> EHLTIGFKVENAHDRILKTIKTHKLKNYIKESVNFLNSGLTKTNYLGSSNDNIELVDFQNIMFYGDAEVGDNQQPFTFILDTGSANLWVPSVKCTTAGCLTKHLYDSSKSRTYEKDGTKVEMNYVSGTVSGFFSKDLVTVGNLSLPYKFIEVIDTNGFEPTYTASTFDGILGLGWKDLSIGSVDPIVVELKNQNKIENALFTFYLPVHDKHTGFLTIGGIEERFYEGPLTYEKLNHDLYWQITLDAHVGNIMLEKANCIVDSGTSAITVPTD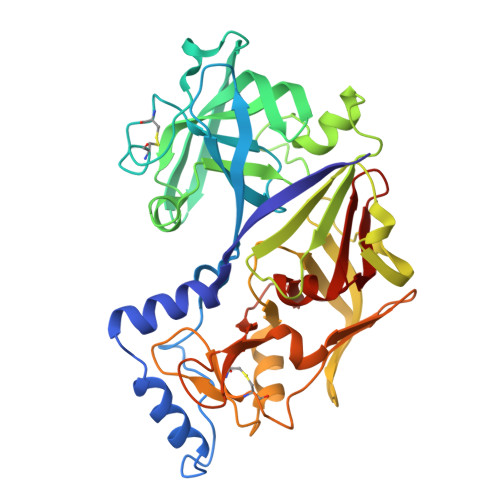FLNKMLQNLDVIKVPFLPFYVTLCNNSKLPTFEFTSENGKYTLEPEYYLQHIEDVGPGLCMLNIIGLDFPVPTFILGDPFMRKYFTVFDYDNHSVGIALAKKNL>[2x]GAMASTEKRLLKEYRAVKKELTEKRSPIHDTGIVDLHPLEDGLFRWSAVIRGPDQSPFEDALWKLEID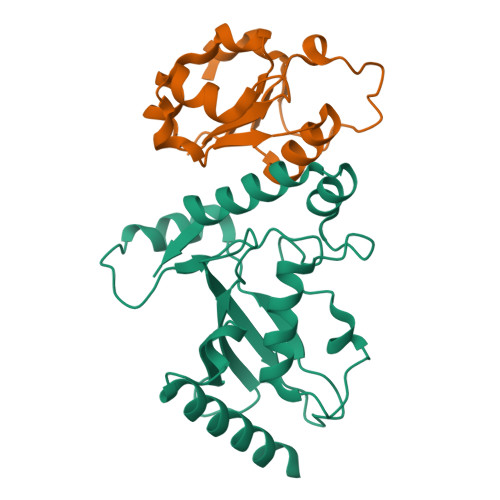IPTNYPLDPPKIKFVVFGEEKIRQLQRKTSSGARKVCYKMPHPNVNFKTGEICLDILQQKWSPAWTLQSALVAIVVLLANPEPLSPLNIDMANLLKCDDTTAYKDLVHYYIAKYSAYESNDV;>GAMAWALKTINPGLFEEPAKTSEASKSNGQSVSLVLTQKDLDFFSAAYLNEYPNLTVILHPSVDKSEFLSRFNVQRNSHQVIQVRTEESIFHVLKQLSSNINLITLGNLEMSANEVETFHLDKFLTNVHEVDRINDYI[2x]>[2x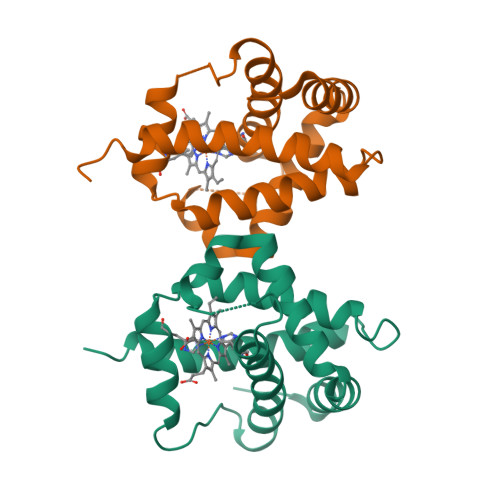]MSFTNVNYPASDGTVIFTEEQEALVVQSWNVMKKNSAELGLKLFLKIFEIAPTAKKMFSFVRDSDVPLEQNQKLKGHAMSVFVMTAKSAAQLRKAGKVTFGESSLKHMGSVHLKYGVVDEHFEVTRFALLETIKEAVPEMWSPEMKNAWAEAFNHLVAAIKAEMQRLSTQP N-{[4-(4-phenylpiperazin-1-yl)oxan-4-yl]methyl}-2-(phenylsulfanyl)pyridine-3-carboxamide 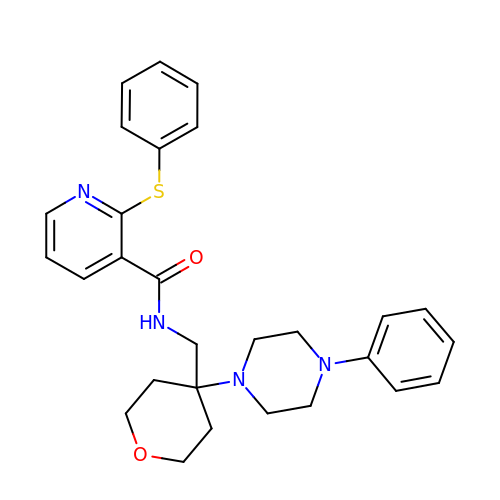| C28 H32 N4 O2 S | XREFXUCWSYMIOG-UHFFFAOYSA-N N-[4-(propan-2-yl)phenyl]pyrazine-2-carboxamide | C14 H15 N3 O | 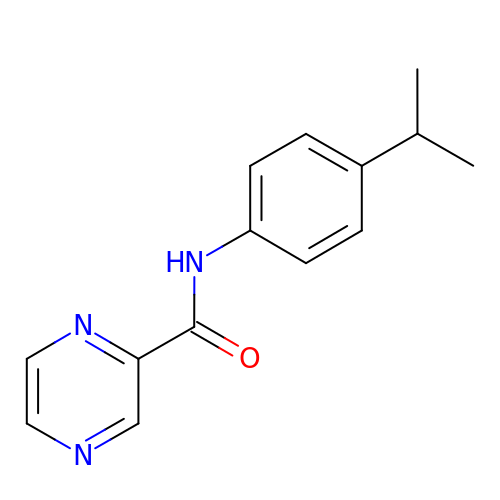REPKUXPMFWYVDC-UHFFFAOYSA-N>SSNDNIELVDFQNIMFYGDAEVGDNQQPFTFILDTGSANLWVPSVKCTTAGCLTKHLYDSSKSRTYEKDGTKVEMNYVSGTVSGFFSKDLVTVGNLSLPYKFIEVIDTNGFEPTYTASTFDGILGLGWKDLSIGSVDPIVVELKNQNKIENALFTFYLPVHDKHTGFLTIGGIEERFYEGPLTYEKLNHDLYWQITLDAHVGNIMLEKANCIVDSGTSAITVPTDFLNKMLQNLDVIKVPFLPFYVTLCNNSKLPTFEFTSENGKYTLEPEYYLQHIEDVGPGLCMLNIIGLDFPVPTFILGDPFMRKYFTVFDYDNHSVGIALAKKN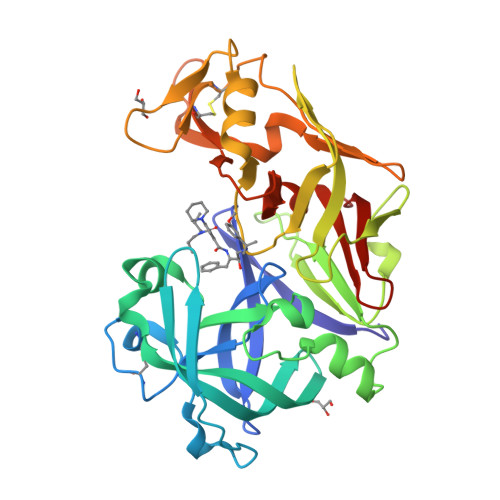L[3x]>ATDRGSESDKHFRKVSDKEKIDQLQEELLHTQLKYQRILERLEKENKELRKLVLQKDDKGIHHRKLKKSLIDMYSEVLDVLSDYDASYNTQDHLPRVVVVGDQSAGKTSVLEMIAQARIFPRGSGEMMTRSPVKVTLSEGPHHVALFKDSSREFDLTKEEDLAALRHEIELRMRKNVKEGCTVSPETISLNVKGPGLQRMVLVDLPGVINTVTSGMAPDTKETIFSISKAYMQNPNAIILCIQDGSVDAERSIVTDLVSQMDPHGRRTIFVLTKVDLAEKNVASPSRIQQIIEGKLFPMKALGYFAVVTGKGNSSESIEAIREYEEEFFQNSKLLKTSMLKAHQVTTRNLSLAVSDCFWKMVRESVEQQADSFKATRFNLETEWKNNYPRLRELDRNELFEKAKNEILDEVISLSQVTPKHWEEILQQSLWERVSTHVIENIYLPAAQTMNSGTFNTTVDIKLKQWTDKQLPNKAVEVAWETLQEEFSRFMTEPKGKEHDDIFDKLKEAVKEESIKRHKWNDFAEDSLRVIQHNALEDRSISDKQQWDAA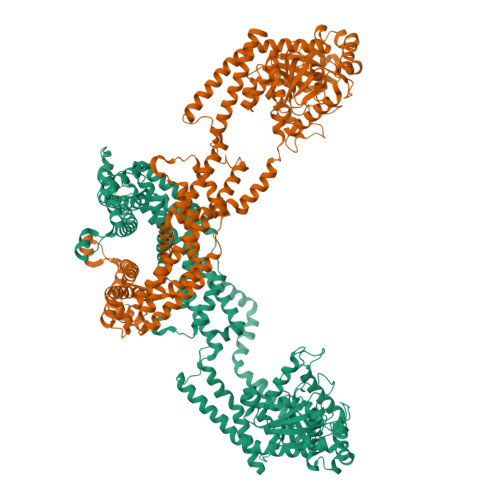IYFMEEALQARLKDTENAIENMVGPDWKKRWLYWKNRTQEQCVHNETKNELEKMLKCNEEHPAYLASDEITTVRKNLESRGVEVDPSLIKDTWHQVYRRHFLKTALNHCNLCRRGFYYYQRHFVDSELECNDVVLFWRIQRMLAITANTLRQQLTNTEVRRLEKNVKEVLEDFAEDGEKKIKLLTGKRVQLAEDLKKVREIQEKLDAFIEALHQEK[2x]>GTSSMADIGSTNDALDYYLKSKGFNGLFSQIELSFSASNLRDRDVLSKSDPMVVVYQKEKDATLSEVFRSEVVLNSLAPKWIKKFIVAYHFETVQTLVFRVYDVDTKFQNSREEMLKLDEQQFLGEATCALSEIITKSTRTSTLELKRKDGFAPQAQPHHGKLIIHAEESLASKISTEIVFRCSNLESKDLFSKSDPFLVVSKIVEHGTPIPVSKTEVRKNDLNPIWKPVFLSVQQVGSKDSPVIIECSDFNSNGKHSLIGKVQKSLSDLEKLHLAGQGINFSLPTGAGQNKVLKSQLFVDKFTETVHHTFLEYLASGFELNFMVAIDFTASNGNPRLPDSLHYIDPSGRLNAYQRAIMDVGEVLQFYDSDKRFPAWGFGARPIDAPVSHCFNLNGSSSYSEVDGIQGIMTSYTSALFNVSLAGPTLFGPVINAAAMIASASLAQGSRKYYVLLIITDGVITDLQETKDALVSASDLPLSILIVGVGGADFKEMEILDADKGERLESSSGRLASRDIVQFVALRDVQYGEISVVQALLAELPSQFLTYMRIRN[4x];> GLFSQIELSFSASNLRDRDVLSKSDPMVVVYQKEKDATLSEVFRSEVVLNSLAPKWIKKFIVAYHFETVQTLVFRVYDVDTKFQNSREEMLKLDEQQFLGEATCALSEIITKSTRTSTLELKRKDGFAPQAQPHHGKLIIHAEESLASKISTEIVFRCSNLESKDLFSKSDPFLVVSKIVEHGTPIPVSKTEVRKNDLNPIWKPVFLSVQQVGSKDSPVIIECSDFNSNGKHSLIGKVQKSLSDLEKLHLAGQGINFSLPTGAGQNKVLKSQLFVDKFTETVHHTFLEYLASGFELNFMVAIDFTASNGNPRLPDSLHYIDPSGRLNAYQRAIMDVGEVLQFYDSDKRFPAWGFGARPIDAPVSHCFNLNGSSSYSEVDGIQGIMTSYTSALFNVSLAGPTLFGPVINAAAMIASASLAQGSRKYYVLLIITDGVITDLQETKDALVSASDLPLSILIVGVGGADFKEMEILDADKGERLESSSGRLASRDIVQFVALRDVQYGEISVVQALLAELPSQFLTYMRIRN;> ADIGSTNDALDYYLKSKGFNGLFSQIELSFSASNLRDRDVLSKSDPMVVVYQKEKDATLSEVFRSEVVLNSLAPKWIKKFIVAYHFETVQTLVFRVYDVDTKFQNSREEMLKLDEQQFLGEATCALSEIITKSTRTSTLELKRKDGFAPQAQPHHGKLIIHAEESLASKISTEIVFRCSNLESKDLFSKSDPFLVVSKIVEHGTPIPVSKTEVRKNDLNPIWKPVFLSVQQVGSKDSPVIIECSDFNSNGKHSLIGKVQKSLSDLEKLHLAGQGINFSLPTGAGQNKVLKSQLFVDKFTETVHHTFLEYLASGFELNFMVAIDFTASNGNPRLPDSLHYIDPSGRLNAYQRAIMDVGEVLQFYDSDKRFPAWGFGARPIDAPVSHCFNLNGSSSYSEVDGIQGIMTSYTSALFNVSLAGPTLFGPVINAAAMIASASLAQGSRKYYVLLIITDGVITDLQETKDALVSASDLPLSILIVGVGGADFKEMEILDADKGERLESSSGRLASRDIVQFVALRDVQYGEISVVQALLAELPSQFLTYMRIRN;> LFSQIELSFSASNLRDRDVLSKSDPMVVVYQKEKDATLSEVFRSEVVLNSLAPKWIKKFIVAYHFETVQTLVFRVYDVDTKFQNSREEMLKLDEQQFLGEATCALSEIITKSTRTSTLELKRKDGFAPQAQPHHGKLIIHAEESLASKISTEIVFRCSNLESKDLFSKSDPFLVVSKIVEHGTPIPVSKTEVRKNDLNPIWKPVFLSVQQVGSKDSPVIIECSDFNSNGKHSLIGKVQKSLSDLEKLHLAGQGINFSLPTGAGQNKVLKSQLFVDKFTETVHHTFLEYLASGFELNFMVAIDFTASNGNPRLPDSLHYIDPSGRLNAYQRAIMDVGEVLQFYDSDKRFPAWGFGARPIDAPVSHCFNLNGSSSYSEVDGIQGIMTSYTSALFNVSLAGPTLFGPVINAAAMIASASLAQGSRKYYVLLIITDGVITDLQETKDALVSASDLPLSILIVGVGGADFKEMEILDADKGERLESSSGRLASRDIVQFVALRDVQYGEISVVQALLAELPSQFLTYMRIR;> GTSSMADIGTTNDALDYYLKSKGFNGLFSQIELSFSASNLRDRDVLSKSDPMVVVYQKEKDATLSEVFRSEVVLNSLAPKWIKKFIVAYHFETVQTLVFRVYDVDTKFQNSREEMLKLDEQQFLGEATCALSEIITKSTRTSTLELKRKDGFAPQAQPHHGKLIIHAEESLASKISTEIVFRCSNLESKDLFSKSDPFLVVSKIVEHGTPIPVSKTEVRKNDLNPIWKPVFLSVQQVGSKDSPVIIECSDFNSNGKHSLIGKVQKSLSDLEKLHLAGQGINFSLPTGAGQNKVLKSQLFVDKFTETVHHTFLEYLASGFELNFMVAIDF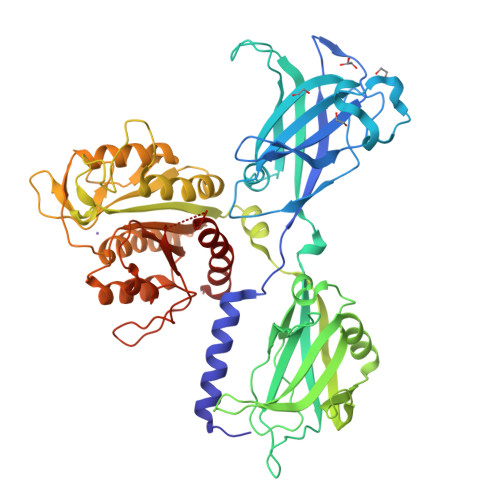TASNGNPRLPDSLHYIDPSGRLNAYQRAIMDVGEVLQFYDSDKRFPAWGFGARPIDAPVSHCFNLNGSSSYSEVDGIQGIMTSYTSALFNVSLAGPTLFGPVINAAAMIASASLAQGSRKYYVLLIITDGVITDLQETKDALVSASDLPLSILIVGVGGADFKEMEILDADKGERLESSSGRLASRDIVQFVALRDVQYGEISVVQALLAELPSQFLTYMRIRN>MGTQKVTPALIFAITVATIGSFQFGYNTGVINAPEKIIKEFIQKTLTDKGNAPPSEVLLTSLWSLSVAIFSVGGMIGSFSVGLFVNRFGRRNSMLIVNLLAVTGGCFMGLCKVAKSVEMLILGRLVIGLFCGLCTGFVPMYIGEISPTALRGAFGTLNQLGIVVGILVAQIFGLEFILGSEELWPLLLGFTILPAILQSAALPFCPESPRFLLINRKEEENAKQILQRLWGTQDVSQDIQEMKDESARMSQEKQVTVLELFRVSSYRQPIIISIVLQLSQQLSGINAVFYYSTGIFKDAGVQEPIYATIGAGVVNTIFTVVSLFLVERAGRRTLHMIGLGGMAFCSTLMTVSLLLKDNYNGMSFVCIGAILVFVAFFEIGPGPIPWFIVAELFSQGPRPAAMAVAGCSNWTSNFLVGLLFPSAAHYLGAYVFIIFTGFLITFLAFTFFKVPETRGRTFEDIT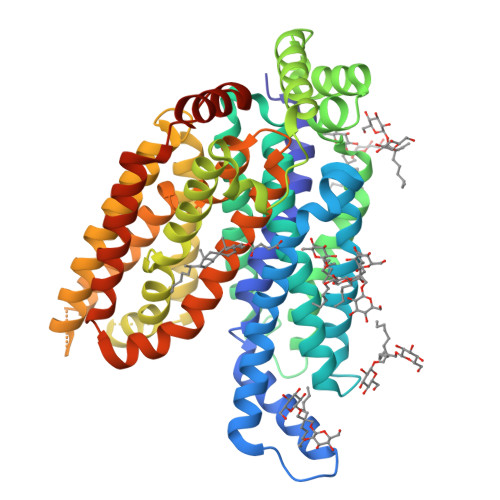RAFEGQAHGADRAENLYFQ[2x]> MRRNRRGSPARPAARFVRPAIPSALSVALLVCTPGLATADPQTDTIAALIADVAKANQRLQDLSDEVQAEQESVNKAMVDVETARDNAAAAEDDLEVSQRAVKDANAAIAAAQHRFDTFAAATYMNGPSVSYLSASSPDEIIATVTAAKTLSASSQAVMANLQRARTERVNTESAARLAKQKADKAAADAKASQDAAVAALTETRRKFDEQREEVQRLAAERDAAQARLQAARLVAWSSEGGQGAPPFRMWDPGSGPAGGRAWDGLWDPTLPMIPS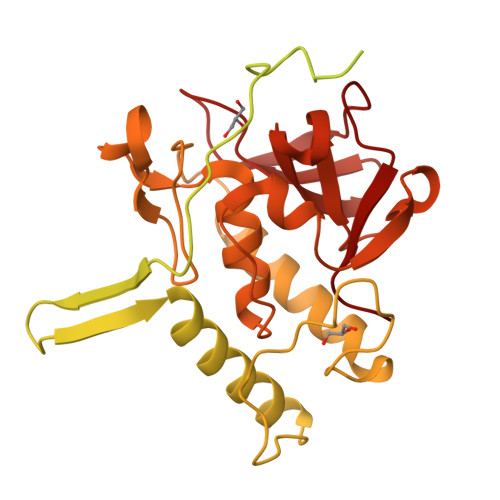ANIPGDPIAVVNQVLGISATSAQVTANMGRKFLEQLGILQPTDTGITNAPAGSAQGRIPRVYGRQASEYVIRRGMSQIGVPYSWGGGNAAGPSKGIDSGAGTVGFDCSGLVLYSFAGVGIKLPHYSGSQYNLGRKIPSSQMRRGDVIFYGPNGSQHVTIYLGNGQMLAAPDVGLKVRVAPVRTAGMTPYVVRYIEY>[4x]MGSSHHHHHHSQDPAPFACVSRWLHTPSFATVSPQEVSGSSPAEVQNFVQGSWTASANWNWIVDPLNGDKFIKVAEVQGTEIKSFMESLSKCPKHGLHNPLKAPERYLMYGDISAKAAHML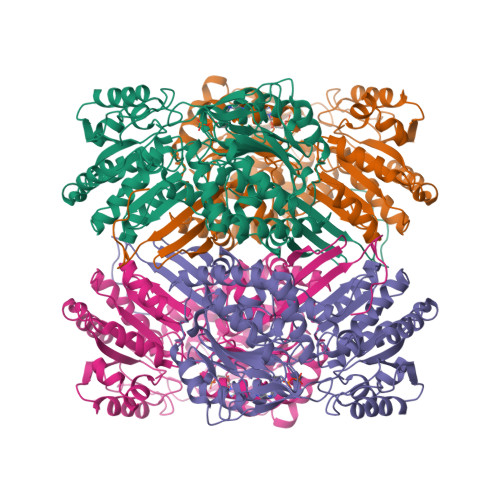GQPTVLDFFAKLIQRVSPKSYQQALAEVQVSQKFLENFCGDQVRFLARSFAVPGNHLGQRSNGYRWPYGPVAIITPFNFPLEIPLLQLMGALYMGNKPVLKVDSKVSIVMEQMIRLLHDCGLPAEDMDFINSDGAVMNKLLLEANPKMTLFTGSSRVAEKLAADLKGRVKLEDAGFDWKILGPDVQEVDYVAWVCDQDAYACSGQKCSAQSVLFMHKNWSSSGLLEKMKKLSERRKLEDLTIGPVLTVTTEAMIEHMNNLLKIRGSKVLFGGEPLANHSIPKIYGAMKPTAVFVPLEEILKSGNFELVTKEIFGPFQVVTEYSEDQLELVLEACERMNAHLTAAIVSNDPLFLQDVLGRSVNGTTYAGIRARTTGAPQNHWFGPAGDPRGAGIGTPEAIKLVWSCHREIIYDVGPVPESWALPSAT We have solved the structure of the prototypic SH2-kinase unit of the human Fes tyrosine kinase, which appears specialized for positive signaling. We investigated the structure of a polypeptide from human Fes comprising a linker region N terminal to the SH2 domain, the SH2 domain, and the C-terminal kinase domain. The three structures were determined in complex with the ATP mimetic kinase inhibitor staurosporine and were refined to low R factors and acceptable geometry. The SH2 domain, the kinase domain, and substrate apparently interact cooperatively to yield a functional Fes kinase complex.

The initial structure of unphosphorylated Fes SH2-kinase revealed an active conformation, which was stabilized by two sulphate ions that mimic binding of a pTyr ligand to the SH2 domain, as well as activation segment phosphorylation. This structure was well ordered, showing productive interactions between the SH2 and kinase domains, and we were able to trace the entire chain; we refer to this structure as “active. In this active configuration, the SH2 domain is stabilized by a sulphate ion, which mimics the phosphate of a pTyr ligand by coordinating a conserved SH2 domain arginine (R483), as well as R467 and S485. In addition, a sulphate ion is coordinated by Y713 and R706 in the activation segment, thereby mimicking autophosphorylation. The SH2 and kinase domains form a stable unit linked by the N-terminal region of the SH2 domain and polar interactions between the SH2 domain helix αA and the catalytically important helix αC. The N terminus of the SH2 domain (462HGAI) intercalates between the central SH2 β sheet and the loop region between strands β4 and β5 in the kinase domain. The second major interaction site is formed by a network of acidic residues located in the SH2 helix αA (E469, E472) and R609 in αC of the kinase. This arrangement suggests that the interaction between the SH2 and kinase domains positions and stabilizes αC in an active conformation, as indicated by the salt bridge formed between the active site lysine (K590) and the conserved αC glutamate (E607), as well as by low B values in loop regions linking this helix. In contrast, the sulphate ion occupying the pTyr-binding site of the SH2 domain in the active Fes structure formed a network of salt bridges typically observed in SH2 domain phosphopeptide complexes, correlating with stabilization and ordering of the SH2 domain and αC. The activation segment in active Fes showed significantly higher temperature factors than in either of the Fes-substrate complexes, indicating the stabilizing effect of substrate binding.

> SMIPEVQKPLHEQLWYHGAIPRAEVAELLVHSGDFLVRESQGKQEYVLSVLWDGLPRHFIIQSLDNLYRLEGEGFPSIPLLIDHLLSTQQPLTKKSGVVLHRAVPKDKWVLNHEDLVLGEQIGRGNFGEVFSGRLRADNTLVAVKSCRETLPPDLKAKFLQEARILKQYSHPNIVRLIGVCTQKQPIYIVMELVQGGDFLTFLRTEGARLRVKTLLQMVGDAAAGMEYLESKCCIHRDLAARNCLVTEKNVLKISDFGMSREEADGVYAASGGLRQVPVKWTAPEALNYGRYSSESDVWSFGILLWETFSLGASPYPNLSNQQTREFVEKGGRLPCPELCPDAVFRLMEQCWAYEPGQRPSFSTIYQELQSIRKRHR> MGSTIEERV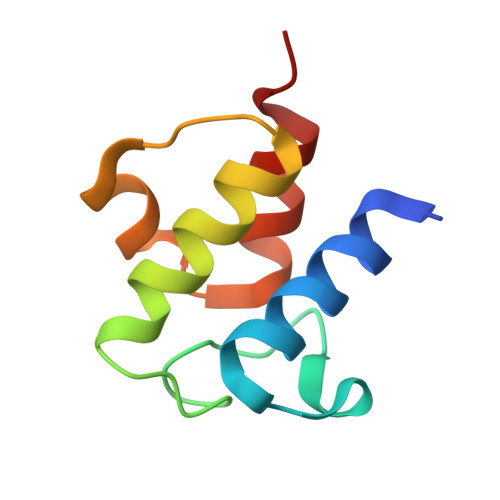KKIIGEQLGVKQEEVTNNASFVEDLGADSLDTVELVMALEEEFDTEIPDEEAEKITTVQAAIDYINGHQA>QMRVNRCIFASIVSFDACITYKSPCSPDAYHDDGWFICNNHLIKRFKMSKMVLPIFDEDDNQFKMTIARHLVGNKERGIKRILIPSATNYQDVFNLNSMMQAEQLIFHLIYNNENAVNTICDNLKYTEGFTSNTQRVIHSVYATTKSILDTTNPNTFCSRVSRDELRFFDVTNARALRGGAGDQLFNNYSGFLQNLIRRAVAPEYLQIDTEELRFRNCATCIIDETGLVASVPDGPELYNPIRSSDIMRSQPNRLQIRNVLKFEGDTRELDRTLSGYEEYPTYVPLFLGYQIINSENNFLRNDFIPRANP[8x]

Baculoviruses are a family of arthropod-infecting, double-stranded DNA viruses. Baculoviruses are insect-infecting pathogens with wide applications as biological pesticides, in vitro protein production vehicles and gene therapy tools. Its cylindrical nucleocapsid, which encapsulates and protects the circular double-stranded viral DNA encoding proteins for viral replication and entry, is formed by the highly conserved major capsid protein VP39. The 39 kDa protein VP39 is the most abundant component of the nucleocapsid, with homologs in alpha- and betabaculoviruses. VP39 forms the capsid shell encasing the nucleocapsid core.

Here, we present a 3.2 Å-resolution electron cryomicroscopy (cryo-EM) structure of the AcMNPV VP39 protein and its assembly into helical nucleocapsids. In our reconstruction, individual VP39 subunits pack as dimers that assemble into 14 helical strands and together form the central cylindrical structure of the baculoviral nucleocapsid. After local alignment, we estimated the overall resolution of the four-dimer reconstruction to be approximately 3.2 Å. We find that the VP39 monomer comprises a distinct mixed alpha/beta fold, which includes a putative Zinc finger domain facing the inside of the nucleocapsid. The Coulomb potential map reveals strong signal in the vicinity of cysteine 18, cysteine 36, cysteine 49, and histidine 52, which are positioned for tetrahedral coordination of a metal ion. Based on the nature and distances of the donor residues, which occur most frequently in Zinc coordination groups, we placed a Zinc metal ion at the center of the coordination group. The ZF faces the luminal volume of the VP39 nucleocapsid assembly and is surrounded by positively charged residues, consistent with a role in binding viral DNA. The intra-dimer interface is stabilized by the 75-residue long lasso loop, parts of which protrude into the adjacent monomer of the repeat domain and wrap around its antenna domain. Using the PDBePISA tool, we identified four inter-dimer contacts, which are all primarily mediated by hydrogen bonding. Lateral contacts stabilizing adjacent units in the nucleocapsid (square symbol) are predicted to be the strongest inter-dimer interactions of the helical assembly (the theoretical total gain in solvation free energy upon interface formation is ΔGsol = −13.8 kcal/mol; obtained from analysis using PDBePISA and defined as the difference in total solvation energies of isolated and interfacing chains).Type IV pili (T4P) are long, thin (5–8 nm diameter) hair-like appendages which extend from the bacterial surface and promote attachment, cell-cell aggregation, biofilm formation, and twitching motility. The T4aP system in P. aeruginosa is composed of four subcomplexes that together form a transenvelope machinery. PilMNOP are critical for function of the T4aP system. PilN and PilO also form heterodimers. They are predicted to have similar topologies, with short cytoplasmic N-termini preceding single transmembrane segments (TMS), followed by periplasmic segments consisting of a coiled-coiled domain linked to a core domain containing two ferredoxin-like αββ motifs.

Although the soluble, stable complex was used for the crystallization experiments, the resulting crystals contained only a truncated form of PilO (PilOΔ109). Although the PilO construct used encompassed residues 52–208, we could model only residues 110–206. PilOΔ109 has two αββ motifs composed of α1-β1β2-β3 and α2-β4β5-β6. The four β-strands form an antiparallel β-sheet onto which the two α-helices pack. Previously, only one discontinuous β-strand was identified in the first αββ motif, but the new structure exhibits another β-strand break in the second αββ motif at the same position, resulting in a secondary structure pattern of α1-β1β2-β3 and α2-β4β5-β6. The main chain carbonyls of D175 and F176 do not participate in hydrogen bonding between the β4β5- and β6-strands in the PilOΔ109 structure, creating the discontinuous β-strand. In the new structure, a dimethyl-Lys residue (K196) was identified on the back face of the β6-strand, the result of the reductive methylation used to promote crystallization of the PilNΔ44/PilOΔ51/PilPΔ18 complex. The monomer orientation in the PilOΔ109 dimer places the β-sheets on the same side, forming a longer 8-stranded anti-parallel β-sheet. Instead, it is more likely that the previously observed PilOΔ68 dimer interface – in which both N- and C-termini are oriented in the same direction, towards the inner membrane – is the biologically relevant one, similar to the orientation described in a recent cryoelectron tomographic model of the T4aP system of M. xanthus. Only PilO R169D and I170A reduced twitching motility (approx. 40% and 50% relative to wild-type, respectively) and levels of surface piliation.

> VPGLLEDITRTGLGSGLEFEEIKLLPEVAQQFYIELPIQISVVGGYHDLATFVSGVSSLPRIVTLHDFEIKPVAPGSTSKLRMSILAKTYRYNDKGLK A BLAST protein sequence alignment search revealed a candidate lectin from Musa acuminata ssp. malaccensis, which we term Malayasian banana lectin (Malay BanLec). Like BanLec, Malay BanLec has a β-prism-I fold characteristic of the jacalin-related lectin family. To assess binding of WT versus F84T to HIV, we conducted surface plasmon resonance analysis to determine the binding times to, and binding avidities for, the gp140 trimer, which is made up of uncleaved ectodomains of the gp160 HIV envelope glycoprotein trimer. The results show that F84T and WT Malay BanLec, which like BanLec exist as dimers with two CBS per monomer (see Fig. 6 below and discussion thereof), bind with high avidity to the gp140 trimer. That is, we asked whether disruption of pi–pi stacking in a structurally related but distinct (only 63% identical at the amino acid level) jacalin-related lectin, Malaysian banana lectin (Malay BanLec), would reduce mitogenicity of the engineered lectin without abolishing antiviral activity.

Between the two CBS, as in wild-type (WT) BanLec, Malay BanLec has a tyrosine at position 83 (Y83), but instead of a histidine at position 84 as in WT BanLec, Malay BanLec has a phenylalanine (F84). First, we aligned the structure of WT Malay BanLec to that of WT BanLec. The structures are remarkably similar, with a root-mean-square deviation (RMSD) between all atoms of only 0.517 Å. However, the aromatic rings involved in pi–pi stacking are arranged in a planar (sandwich) conformation in BanLec, whereas they are arranged in an edge-on conformation in Malay BanLec. Malay BanLec treatment resulted in greater BrdU incorporation than did WT BanLec treatment at concentrations up to 10 nM, but less incorporation above that concentration, which may be due to cell death triggered by excessive mitogenic stimulation. These results indicate that Malay BanLec is indeed mitogenic, and highly so as it is even more stimulatory than WT BanLec. Therefore, Malay BanLec, like WT and H84T BanLec, does possess antiviral activity and perhaps has more potent activity against certain strains of HIV than does either WT or H84T BanLec. We would expect Y83 and F84 in Malay BanLec to interact via pi–pi stacking. Thus, although Malay BanLec is quite a different lectin than BanLec with only 63% amino acid identity (differing at 52 of 141 amino acids), it is predicted to have important structural features in common with BanLec that make it a suitable candidate to engineer in a similar fashion, with a view to reducing mitogenicity while retaining antiviral activity.

>[2x]MAGAIKVGTWGGNGGSEWDMGPAYRIDSVKINAGDIIDAIEITFTRYGLTETQHYGGTGGEPHEIAFEDGEYIMSMEGHVVDYFGLTIIGKLTLTTNRRTFGPFGAYEGTPFSIPVAEGKIAGFFGRAGSFIDAIGVYLMPNLEHHHHHH>[4x]MEQQLKDIISACDLAIQNEDFDTLMNYYSEDAVLVVKPGMIARGKEEIKKAFITIAN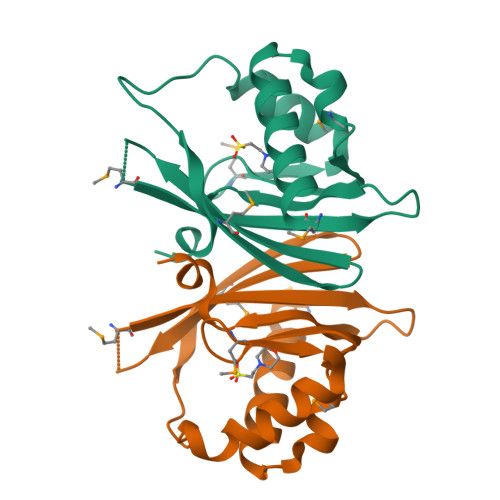YFNHHIVPTQGKMILLEAGDTVLVLSQTLLDSDKKDSEYAMERRATYVFKKNAQGEWLCVIDNSYGTDLIGVMAGDPLEHHHHHH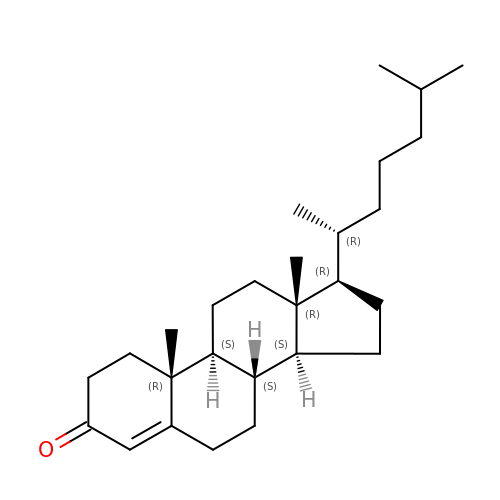(8ALPHA,9BETA)-CHOLEST-4-EN-3-ONE | C27 H44 O | NYOXRYYXRWJDKP-GYKMGIIDSA-N4-(4-FLUORO-PHENYLAZO)-5-IMINO-5H-PYRAZOL-3-YLAMINE | C9 H7 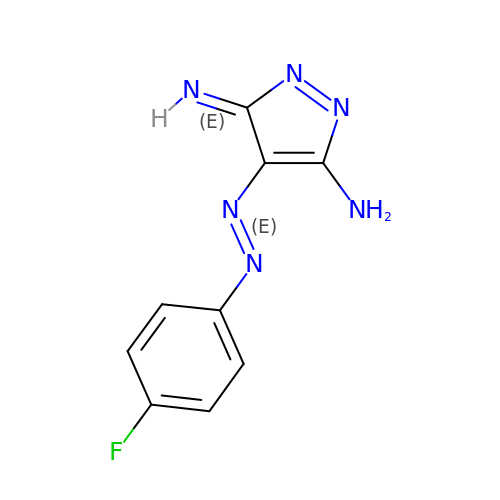F N6 | HALOLQDLOLYIOW-ZOBWXTBZSA-N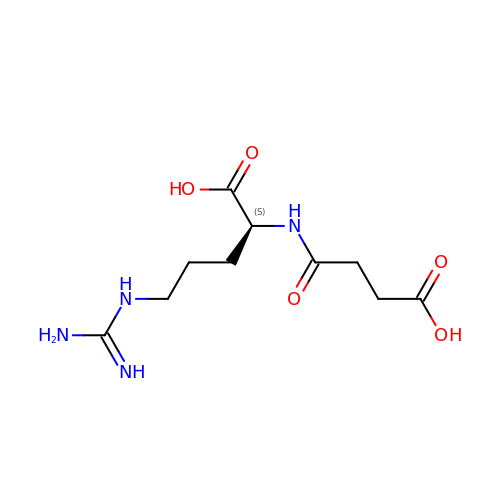N~2~-(3-CARBOXYPROPANOYL)-L-ARGININE | C10 H18 N4 O5 | UMOXFSXIFQOWTD-LURJTMIESA-N The Lon protease is a AAA+ protein found in prokaryotes, archaea, and eukaryotic organelles. Lon is involved in cellular protein homeostasis by degrading damaged or misfolded abnormal proteins, which prevents these unwanted protein species from forming toxic aggregates. Lon is known to form a homohexamer; each protomer is composed of multiple domains, including an N-terminal substrate-binding globular domain (NGD), a long-helix domain (LH), a three-helix bundle (3H), a AAA+ ATPase module, and a protease domain. We show here, using cryo-electron microscopy (cryo-EM), that the activation process of the Lon AAA+ protease may involve a pentameric assembly and a substrate-dependent incorporation of the sixth protomer to form the substrate-pore-loop contacts seen in the translocating state.

To provide a comparative context, we also examined wild-type MtaLon in two states: without any nucleotide (MtaLon-Apo) and incubated with 5 mM ADP (MtaLon:ADP). Additionally, our cryo-EM structures of a series of spiral subcomplex oligomers of Lon determined by 3D reconstructions suggest a sequential pathway for the construction of the THT. In the proposed pathway, the THT is formed by sequential incorporation of the protomers, beginning with Ob1 and progressing in the clockwise direction through Ob5, and completed by the incorporation of Ac6*, whose binding mode is dependent on the substrate.

>[4x]MRLELPVIPLRNTVILPHTTTPVDVGRAKSKRAVEEAMGADRLIFLVAQRDPEVDDPAPDDLYTWGVQAVVKQAMRLPDGTLQVMVEARARAQVTDYIPGPYLRARGEVFSEIFPIDEAVVRVLVEELKEAFEKYVANHKSLRLDRYQLEAVKGTSDPAMLADTIAYHATWTVAEKQEILELTDLEARLKKVLGLLSRDLERFELDKRVAQRVKEQMDTNQREYYLREQMKAIQKELGGEDGLSDLEALRKKIEEVGMPEAVKTKALKELDRLERMQQGSPEATVARTYLDWLTEVPWSKADPEVLDINHTRQVLDEDHYGLKDVKERILEYLAVRQLTQGLDVRNKAPILVLVGPPGVGKTSLGRSIARSMNRKFHRISLGGVRDEAEIRGHRRTYIGAMPGKLIHAMKQVGVINPVILLDEIDKMSSDWRGDPASAMLEVLDPEQNNTFTDHYLDVPYDLSKVFFITTANTLQTIPRPLLDRMEVIEIPGYTNMEKQAIARQYLWPKQVRESGMEGRIEVTDAAILRVISEYTREAGVRGLERELGKIARKGAKFWLEGAWEGLRTIDASDIPTYLGIPRYRPDKAETEPQVGTAQGLAWTPVGGTLLTIEVAAVPGSGKLSLTGQLGEVMKESAQAALTYLRAHTQDYGLPEDFYNKVDLHVHVPDGATPKDGPSAGITMATAIASALSRRPARMDIAMTGEVSLRGKVMPIGGVKEKLLAAHQAGIHKIVLPKDNEAQLEELPKEVLEGLEIKLVEDVGEVLEYLLLPEPTMPPVVQPSDNRQQPGAGA> MSKLISPAELAKRLSSKETKIFDATWYLPTPANVGKNAYDNYMKKRIPGALYFDIDAVNTPSK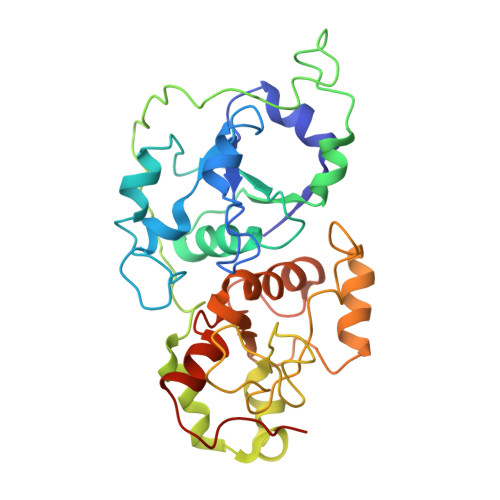FPHMLPSPQTFENELTKLGVSSDSPIVVYDTQGVFSGPRLVWTFKVFGHDNVQFLNGFEAYTQLPGIPSRPDAYTWGIWDTQVPGKIDPADPPYKVTKARPELVKSFEDVLAIVEKHNGDGAKIRNEVTFIDARPNGRFTGKDAEPRAELSSGHVPGAYSIAFPEVVENGKFKSPEELKALFASKGIDGSKPIISMCGSGVTACVIDLALEIAGIGSRDTNAVYDGSWTEWAQRAPTKYIVKEENLNEANRA> LPVNTRCKLHVRNFQSPYIVNRTFMLAKEASLADQNTDVRLIGEKLFRGVSAKDQCYLMKQVLQFTLEDVLLPQSDRFQPYMWEVVPFLTKLSNKL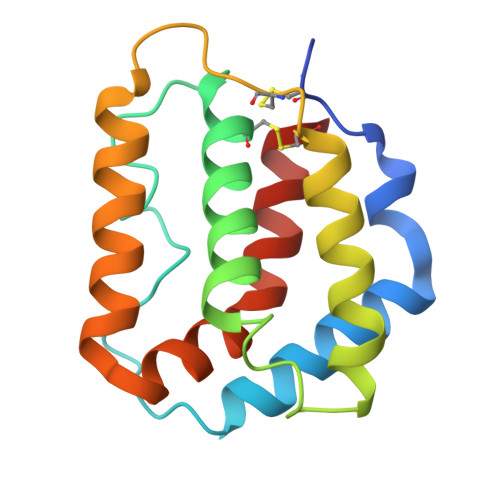SSCHISGDDQNIQKNVRRLKETVKKLGESGEIKAIGELDLLFMSLRNACVGGS>[3x]SQQLQKEEEARKVKSGIRQMRLFSQDECAKIEARIDEVVSRAEKGLYNEHTVDRAPLRNKYFFGEGYTYGAQLQKRGPGQERLYPPGDVDEIPEWVHQLVIQKLVEHRVIPEGFVNSAVINDYQPGGCIVSHVDPIHIFERPIVSVSFFSDSALCFGCKFQFKPIRVSEPVLSLPVRRGSVTVLSGYAADEITHCIRPQDIKERRAVIILRKTRLDAPRL

AlkB homologue 5 (ALKBH5) is a ferrous iron and 2-oxoglutarate dependent oxygenase that demethylates RNA N6-methyladenosine (m6A), a post-transcriptional RNA modification with an emerging set of regulatory roles. We report three crystal structures of ALKBH5 in complex with an m6A-ssRNA 8-mer substrate and supporting biochemical analyses. Strikingly, the single-stranded RNA substrate binds to the active site of ALKBH5 in a 5′-3′ orientation that is opposite to single-stranded or double-stranded DNA substrates observed for other AlkB subfamily members, including single-stranded DNA bound to FTO. The results support a mechanism involving formation of an m6A hemiaminal intermediate, followed by efficient ALKBH5 catalyzed demethylation, enabled by a proton shuttle network involving Lys132 and Tyr139.

Using higher ligand concentrations in the sample mixture and the crystallization drops, we subsequently determined structures of (i) ALKBH574–292 in complex with the same m6A-containing 8-mer ssRNA and the 2OG cosubstrate in the P32 crystal form to 2.1 Å resolution, and (ii) a structure of ALKBH574–292 in complex with NOG and the m6A-containing 8-mer ssRNA in the P21 crystal form to 2.5 Å resolution. The three structures from both crystal forms manifest similar overall protein conformations among molecules in the asymmetric unit of each structure, and when compared among the three structures using Chain A from each structure as representatives (RMSDs Cα 0.2 Å (Chain A from the ALKBH574–292–NOG–RNA complex) and 0.2 Å (Chain A from the ALKBH574–292-RNA complex) relative to Chain A from the ALKBH574–292–2OG–RNA complex). At the ALKBH5 active site in the structures reported here, a catalytically inert Mn ion (substituting for catalytically active Fe(II)) is coordinated by the highly conserved metal binding triad His204, Asp206, and His266, a water molecule, and either 2OG, NOG, or a sulfate ion. The C-5 carboxylate group of 2OG is positioned to form a salt bridge with the side chain of Arg277. The 2OG ketone oxygen and one of the 2OG C-1 carboxylate oxygens chelate to the metal in a bidentate manner and form a hydrogen bond and electrostatic interactions with the side chains of Asn193 and Arg283, respectively. The crystallographically observed 2OG and NOG binding modes in ALKBH5 when complexed with Mn and an m6A substrate are of the ‘off-line’ mode. In the ALKBH574–292-2OG-substrate complex, the N6-methyl group of m6A is positioned ∼4.0 Å away from the Mn, a substrate-metal distance consistent with a (near) catalytically productive orientation as observed in other structures of 2OG oxygenase enzyme-substrate complexes. The phenolic hydroxyl of Tyr139 is positioned to form a hydrogen bond with N6 of m6A, and with Lys132.> CG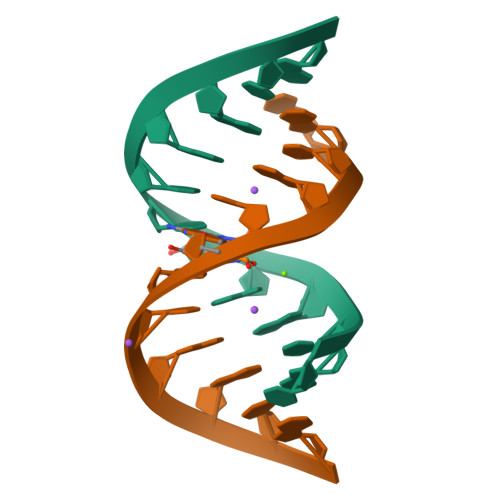CGAAUUAGCG> GSPESFPDAHMRMILRKPPGQRTVDDLEIIYDELLHIKALSHLSTTVKRELAGVLIFESHAKGGTVLFNQGEEGTSWYIILKGSVNVVIYGKGVVCTLHEGDDFGQLALVNDAPRAASIVLREDNCHFLRVDKEDFNRILRDVEANTVRLKEHDQDVLVLEKVPAGNRAANQGNSQPQQKYTVMSGTPEKILEHFLETIRLEPSLNEATDSVLNDFVMMHCVFMPNTQLCPALVAHYHAQPSQGTEQERMDYALNNKRRVIRLVLQWAAMYGDLLQEDDVAMAFLEEFYVSVSDDARMMAAFKEQLPELEKIVKQISEDAKAPQKKHKVLLQQFNTGDERAQKRQPIRGSDEVLFK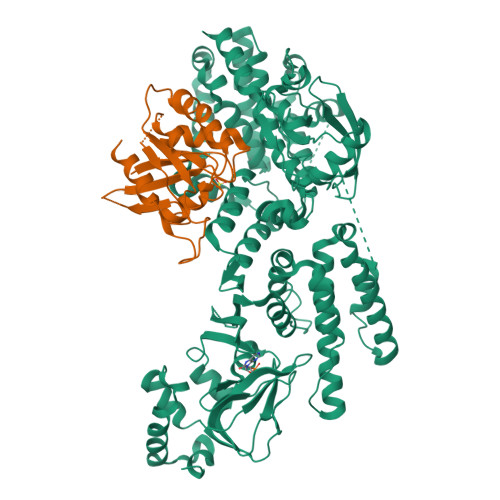VYCIDHTYTTIRVPVAASVKEVISAVADKLGSGEGLIIVKMNSGGEKVVLKSNDVSVFTTLTINGRLFACPREQFDSLTPLPEQEGPTTGTVGTFELMSSKDLAYQMTTYDWELFNCVHELELIYHTFGRHNFKKTTANLDLFLRRFNEIQFWVVTEVCLCSQLSKRVQLLKKFIKIAAHCKEYKNLNSFFAIVMGLSNVAVSRLALTWEKLPSKFKKFYAEFESLMDPSRNHRAYRLTAAKLEPPLIPFMPLLIKDMTFTHEGNKTFIDNLVNFEKMRMIANTARTVRYYRSQPFNPDAAQANKNHQDVRSYVRQLNVIDNQRTLSQMSHRLEPRRP;> MREYKLVVLGSGGVGKSALTVQFVQGIFVEKYDPTIEDSYRKQVEVDAQQCMLEILDTAGTEQFTAMRDLYMKNGQGFALVYSITAQSTFNDLQDLREQILRVKDTDDVPMILVGNKCDLEDERVVGKEQGQNLARQWNNCAFLESSAKSKINVNEIFYDLVRQINR> MAGHTQQPSGRGNPRPAPSPSPVPGTVPGASERVALKKEIGLLSACTIIIGNIIGSGIFISPKGVLEHSGSVGLALFVWVLGGGVTALGSLCYAELGVAIPKSGGDYAYVTEIFGGLAGFLLLWSAVLIMYPTSLAVISMTFSNYVLQPVFPNCIPPTTASRVLSMACLMLLTWVNSSSVRWATRIQDMFTGGKLLALSLIIGVGLLQIFQGHFEELRPSNAFAFWMTPSVGHLALAFLQGSFAFSGWNFLNYVTEEMVDARKNLPRAIFISIPLVTFVYTFTNIAYFTAMSPQELLSSNAVAVTFGEKLLGYFSWVMPVSVALSTFGGINGYLFTYSRLCFSGAREGHLPSLLAMIHVRHCTPIPALLVCCGATAVIMLVGDTYTLINYVSFINYLCYGVTILGLLLLRWRRPALHRPIKVNLLIPVAYLVFWAFLLVFSFISEPMVCGVGVIIILTGVPIFFLGVFWRSKPKCVHRLTESMTHWGQELCFVVYPQDAPEEEENGPCPPSLLPATDKPSKPQ;> MELQPPEASIAVVSIPRQLPGSHSEAGVQGLSAGDDSELGSHCVAQTGLELLASGDPLPSASQNAEMIETGSDCVTQAGLQLLASSDPPALASKNAEVTGTMSQDTEVDMKEVELNELEPEKQPMNAASGAAMSLAGAEKNGLVKIKVAEDEAEAAAAAKFTGLSKEELLKVAGSPGWVRTRWALLLLFWLGWLGMLAGAVVIIVRAPRCRELPAQKWWHTGALYRIGDLQAFQGHGAGNLAGLKGRLDYLSSLKVKGLVLGPIHKNQKDDVAQTDLLQIDPNFGSKEDFDSLLQSAKKKSIRVILDLTPNYRGENSWFSTQVDTVATKVKDALEFWLQAGVDGFQVRDIENLKDASSFLAEWQNITKGFSEDRLLIAGTNSSDLQQILSLLESNKDLLLTSSYLSDSGSTGEHTKSLVTQYLNATGNRWCSWSLSQARLLTSFLPAQLLRLYQLMLFTLPGTPVFSYGDEIGLDAAALPGQPMEAPVMLWDESSFPDIPGAVSANMTVKGQSEDPGSLLSLFRRLSDQRSKERSLLHGDFHAFSAGPGLFSYIRHWDQNERFLVVLNFGDVGLSAGLQASDLPASASLPAKADLLLSTQPGREEGSPLELERLKLEPHEGLLLRFPYAA

The amino acid transporter Asc1/CD98hc (SLC7A10/SLC3A2) is a non-stereoselective small neutral amino acid exchanger (e.g., glycine and, L- and D-serine, alanine, cysteine, and threonine)1–4 expressed mainly in the brain and adipose tissue. Asc1/CD98hc belongs to the family of Heteromeric Amino acid Transporters (HATs), which are composed of a transporter (SLC7; L-amino acid transporter; LAT) and an ancillary (SLC3) subunit linked by a disulfide bridge. Interestingly, Asc1/CD98hc is the only HAT for neutral amino acids that is not an obligatory exchanger, and it also mediates the release of intracellular substrates by facilitated diffusion. Asc1/CD98hc is also the only member of the HAT family that efficiently transports glycine, and D- and L-enantiomers of the amino acid serine, and this particular substrate selectivity underlies the physiological functions of this transporter in both the central nervous system and adipose tissue.

We determined the structure of the human Asc1/CD98hc heterodimer in the absence of substrate in an inward-open conformation with a partial occlusion of TM1a, as described in detail below. We further classified the dataset by using iterative 3D reconstructions and classifications to yield a subset of particles that were refined to high resolution by removing the contribution of noise from the micelle using non-uniform refinement. The estimated average resolution for the cryoEM map of Asc1/CD98hc was ~ 4 Å, with local resolutions as good as 3.4–3.8 Å for most of the map, except for some flexible cytoplasmic regions, thereby allowing the modeling of the Asc1/CD98hc heterodimer structure. The structure of the heterodimer was confidently modeled for residues 41–489 for Asc1 and 61–529 for CD98hc, thus excluding the flexible N-terminal ends of both proteins. Asc1 is covalently bound to CD98hc via a disulfide bridge involving residues Cys 154 (Asc1) and Cys 109 (CD98hc), with additional contacts between CD98hc TM’ helix and the surrounding TM helices of Asc1. The four N-glycosylation sites of CD98hc (residues 264, 280, 323, and 405) were also modeled. Finally, density for a digitonin molecule was observed near TM helices 3, 9, 10, and 12, as previously reported for human LAT221. The substrate binding site of the human Asc1 transporter is in an inward-facing partially occluded conformation, with TM1a tilted to limit the access of substrates to the binding site from the cytosolic side of the membrane. The semi-occlusion of Asc1 is the result of a partial tilting of TM1a to an intermediate position between the fully open cytosolic gate of human LAT221 and the fully occluded cytosolic gate of human LAT125.>GPGSILNFIIDSSSFEKGLGNIAIWSKLNDPKLTINAYLPLFTIQELDFQRFKRKSVVAKRALHFIDLLQDSTSFKLHLEYPELNEAISWNETVKLCQQNSHTSLSQHQISVIPIRFKKLLKSCYYKCHYKSHDLDEDIDHTNEKSDPDDKGWVLVTEDDTVRSLATQFQIPFISVVEADAIINACIKDKSY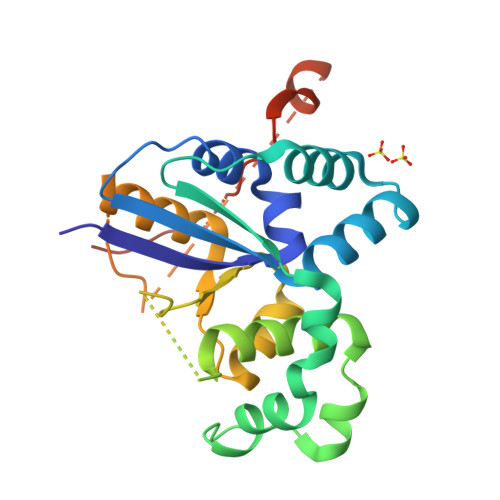VVNEKFSKTVIKKANKVKEQEDGKKVFVTXXXXXDFKNDFLAPRAKSGELWTPTSAKNKS[2x]>ELPNYLVTLPARLNFPSVQKVCLDLSPGYSDVKFTVTLETKDKTQKLLEYSGLKKRHLHCISFLVPPPAGGTEEVATIRVSGVGNNISFEEKKKVLIQRQGNGTFVQTDKPLYTPGQQVYFRIVTMDSNFVPVNDKYSMVELQDPNSNRIAQWLEVVPEQGIVDLSFQLAPEAMLGTYTVAVAEGKTFGTFSVEEYVLPKFKVEVVEPKELSTVQESFLVKICCRYTYGKPMLGAVQVSVCQKANTYWYREVEREQLPDKCRNLSGQTDKTGCFSAPVDMATFDLIGYAYSHQINIVATVVEEGTGVEANATQNIYISPQMGSMTFEDTSNFYHPNFPFSGKIRVRGHDDSFLKNHLVFLVIYGTNGTFNQTLVTDNNGLAPFTLETSGWNGTDVSLEGKFQMEDLVYNPEQVPRYYQNAYLHLRPFYSTTRSFLGIHRLNGPLKCGQPQEVLVDYYIDPADASPDQEISFSYYLIGKGSLVMEGQKHLNSKKKGLKASFSLSLTFTSRLAPDPSLVIYAIFPSGGVVADKIQFSVEMCFDNQVSLGFSPSQQLPGAEVELQLQAAPGSLCALRAVDESVLLLRPDRELSNRSVYGMFPFWYGHYPYQVAEYDQCPVSGPWDFPQPLIDPMPQGHSSQRSIIWRPSFSEGTDLFSFFRDVGLKILSNAKIKKPVDCSHRSPEYSTAMGAGGGHPEAFESSTPLHQAEDSQVRQYFPETWLWDLFPIGNSGKEAVHVTVPDAITEWKAMSFCTSQSRGFGLSPTVGLTAFKPFFVDLTLPYSVVRGESFRLTATIFNYLKDCIRVQTDLAKSHEYQLESWADSQTSSCLCADDAKTHHWNITAVKLGHINFTISTKILDSNEPCGGQKGFVPQKGRSDTLIKPVLVKPEGVLVEKTHSSLLCPKGKVASESVSLELPVDIVPDSTKAYVTVLGDIMGTALQNLDGLVQMPSGCGEQNMVLFAPIIYVLQYLEKAGLLTEEIRSRAVGFLEIGYQKELMYKHSNGSYSAFGERDGNGNTWLTAFVTKCFGQAQKFIFIDPKNIQDALKWMAGNQLPSGCYANVGNLLHTAMKGGVDDEVSLTAYVTAALLEMGKDVDDPMVSQGLRCLKNSATSTTNLYTQALLAYIFSLAGEMDIRNILLKQLDQQAIISGESIYWSQKPTPSSNASPWSEPAAVDVELTAYALLAQLTKPSLTQKEIAKATSIVAWLAKQHNAYGGFSSTQDTVVALQALAKYATTAYMPSEEINLVVKSTENFQRTFNIQSVNRLVFQQDTLPNVPGMYTLEASGQGCVYVQTVLRYNILPPTNMKTFSLSVEIGKARCEQPTSPRSLTLTIHTSYVGSRSSSNMAIVEVKMLSGFSPMEGTNQLLLQQPLVKKVEFGTDTLNIYLDELIKNTQTYTFTISQSVLVTNLKPATIKVYDYYLPDEQATIQYSDPCE[2x]

Human alpha-2 macroglobulin-like 1 (A2ML1) is a monomeric member of the A2M superfamily (A2MF) of protease inhibitors and complement factors. The functional inhibitory unit of A2ML1 is a monomer that depends on covalent binding of the protease (mediated by A2ML1’s thioester) to achieve inhibition. A2MF protease inhibitors utilize a unique trapping mechanism that pseudo-inhibits proteases regardless of their catalytic class. Trapped proteases remain catalytically active but are prevented from cleaving protein substrates through steric hindrance imposed by the inhibitor following a proteolytically triggered conformational change.

Structures of native A2ML1 were determined by X-ray crystallography and cryo-EM at resolutions of 4.4 and 3.1 Å, respectively. An initial crystallographic map was obtained by molecular replacement with a map excised from an early stage cryo-EM map with a resolution of 3.8 Å. Density modification with 70% solvent and two-fold averaging resulted in an outstanding electron density for the X-ray structure in many regions despite the resolution. Overall, the cryo-EM and X-ray structures are very similar with an overall root mean square deviation (RMSD) of 2.0 Å for the entire molecule. Multiple regions in the α-helical TE domain appeared to have better electron density in the X-ray structure than in the EM map, and the Gln1175-Glu1188 loop could only be modeled in this map. These differences in loop flexibility are likely to be an effect of crystal packing interactions involving the TE domain. While the CTM8 body shows minor overall differences between the X-ray and the EM structures, the orientations of the MG3 and MG4 domains within the MG-ring differ significantly due to crystal packing interactions. In both the EM and the X-ray structures of native A2ML1, it is not possible to model residues His696-Asp726, suggesting substantial flexibility of the intact bait region in accordance with its accessibility toward proteases. However, in both structures, it is evident that the strictly conserved residues Arg730-Pro734 pass through the same narrow opening that houses the Nt-α′ in complement A2MF proteins.> GSHMASMKKKGSVVIVGRINLSGDTAYAQQTRGEEGCQETSQTGRDKNQVEGEVQIVSTATQTFLATSINGVLWTVYHGAGTRTIASPKGPVTQMYTNVDKDLVGWQAPQGSRSLTPCTCGSSDLYLVTRHADVIPVRRRGDSRGSLLSPRPISYLKGSAGGPLLCPAGHAVGIFRAAVSTRGVAKAVAFIPVESLETTMRSP

The HCV NS3/4A protease – a chymotrypsin-like serine protease – is a prime therapeutic target that cleaves four known sites along the virally encoded polyprotein. The NS3/4A protease also hydrolyzes two human proteins, TRIF and MAVS, which are part of the innate immune system, thereby confounding the innate immune response to viral infection. In this study, we report that four chemically representative protease inhibitors – telaprevir, danoprevir, vaniprevir and MK-5172 – exhibit distinct susceptibilities to the protease variants R155K, A156T and D168A. To elucidate the underlying mechanism by which chemically diverse inhibitors bind to the wild-type protease and drug-resistant variants, crystal structures were determined for 16 inhibitor-protease complexes. These complexes include wild-type protease and resistant variants R155K, D168A and A156T each bound to telaprevir, danoprevir, vaniprevir and MK-5172, with resolutions ranging from 1.10–2.50 Å; S139A protease variants were used except for telaprevir, which requires covalent bond formation with the serine 139 for efficient binding.

Telaprevir potency was slightly better against D168A relative to the wild type, while danoprevir, vaniprevir and MK-5172 lost 100- to 1000-fold potency against D168A. Among the macrocyclic drugs, danoprevir and MK-5172 retained higher activities against D168A (D168A IC50 = 48 nM and 13 nM, respectively) relative to vaniprevir (D168A IC50>400 nM). The D168A mutation also disrupted stacking of the P2 moieties with R155, by disrupting the electrostatic network and therefore the position of R155 for optimal cation-π stacking. In danoprevir, the P2 isoindoline moiety shifted in response to R155K and D168A mutations, making extensive interactions with the catalytic D81. Thus, D168A caused losses in danoprevir and vaniprevir potency by disrupting cation-π stacking. However, the flexibility of the P2 moiety of danoprevir compensates somewhat for this loss, explaining danoprevir's greater potency against the D168A variant relative to vaniprevir. Interestingly, while both drugs lose considerable potency against R155K, danoprevir retains higher activity against D168A. This difference is likely due to the flexible P2 isoindoline moiety of danoprevir, which lacks P2–P4 cyclization and repacks against the D168A variant. Danoprevir's isoindoline moiety bound in two conformations in the wild-type complex, but adopted a single conformation in mutant complexes. The flexible P2 isoindoline moiety of danoprevir containing a P1–P3 macrocycle packs against the mutated surfaces of A156T and D168A variants, explaining its relatively higher activity against both protease variants.> IVGGYTCAANSIPYQVSLNSGSHFCGGSLINSQWVVSAAHCYKSRIQVRLGEHNIDVLEGNEQFINAAKIITHPNFNGNTLDNDIMLIKLSSPATLNSRVATVSLPRSCAAAGTECLISGWGNTKSSGSSYPSLLQCLKAPVLSDSSCKSSYPGQITGNMICVGFLEGGKDSCQGDSGGPVVCNGQLQG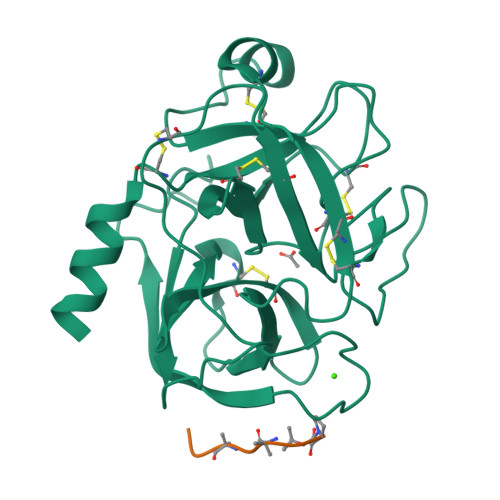IVSWGYGCAQKNKPGVYTKVCNYVNWIQQTIAAN;> PDALALA> MQKHNEDLKESFLLFDGDGDGYLTLNEFESLVRVLGVVMETSAIASTYNSNSKVRGMSYELFTSCFSQLKTKSFNKDEIKTAINVLDKDKKGFIPAIELRRILSTIGDNMEQKEITDLFTFMGIDEQGVVKVDDFINQDNHHHHHH

EhCaBP5 is one of the EF hand calcium-binding proteins of E. histolytica. Sequence analysis of the calcium binding protein 5 from E. histolytica (EhCaBP5) indicates that its size (16.3 kDa) and secondary structural arrangement are similar to those of CaM like proteins but it also suggests the presence of two calcium binding loops in two separate lobes. The overall structure of EhCaBP5 is more similar to that of the essential light chain (ELC) of myosin than to CaM. Taken together, our structural studies show that EhCaBP5 resembles ELCs, and the functional studies indicate that it is likely to be the ELC of myosin 1B.

We have determined the crystal structure of EhCaBP5 at 1.9 Å resolution in the Ca2+-bound state, which shows an unconventional mode of Ca2+ binding involving coordination to a closed yet canonical EF-hand motif. The final refined structure contains 131 residues, one calcium ion, 40 waters and 3 acetates; six residues from the N-terminus could not be modelled due to missing electron density. Overall, the molecule is divided in two globular lobes, where each lobe has four alpha helices connected by loops. The N-terminal lobe has one EF-hand motif with a calcium ion bound to the loop between two helices. Taken together, these results suggest that the C-terminal lobe of EhCaBP5 cannot bind Ca2+. In EhCaBP5, the Ca2+ is coordinated by one carboxyl oxygen each of residues Asp16, Asp18, and Asp20, the hydroxyl oxygen of Tyr22, and two water molecules (instead of one, as observed in CaM). The extra water also binds to the 12th position glutamate of the EF hand loop; this residue is usually critical in directly coordinating Ca2+, but, in EhCaBP5, it is too far away, at a distance of about 4.1 Å, and cannot directly coordinate instead it coordinates the Ca2+ via the intervening water molecule. Overall, the Ca2+coordination geometry is octahedral in EhCaBP5, instead of being pentagonal bipyramidal as is typically found in CaM. The r.m.s.d. between these EF-hand motifs is indeed relatively large, at 2.38 Å, and the interhelical angles of the EF-hand motifs of EhCaBP5 and CaM are 64.3 degrees and 89.3 degrees respectively, indicative of the closed and open conformations respectively. The extensive hydrophobic interaction between these two helices could be the reason for the observed closed state of the lobe and water mediated Ca2+coordination or intermediate state in EhCaBP5.High mobility group (HMG) proteins are intrinsically disordered nuclear non-histone chromosomal proteins that play an essential role in many biological processes by regulating the expression of numerous genes in eukaryote cells. HMGA proteins contain three DNA binding motifs, the “AT-hooks”, that bind preferentially to AT-rich sequences in the minor groove of B-form DNA. The AT-hook motif is formed by a short stretch of amino acids containing a conserved core sequence, Arg-Gly-Arg-Pro (R-G-R-P), flanked by other positively charged amino acids. HMGA are abundant nonhistone architectural nuclear factors that are involved in the modulation of chromatin structure and gene expression, thus influencing a vast array of biological processes including growth, proliferation, differentiation and death.

In the present study, we elucidate the crystal structure of the complex of AT-hook 1 (KRGRGRPRK) with the DNA oligonucleotide d(CGTTAATTAACG)2 at 1.40 Å resolution. Four Mg ions also contribute to stabilize the crystal structure. The terminal bases of the dodecamers do not form Watson-Crick base pairs; instead, the terminal guanines occupy an external position and form N2-N3 hydrogen bonds with the guanines from a neighbour stacked duplex. Peptide G is fully visible in the structure. It has the conformation expected for an AT-hook; its R3-G4 region enters into the minor groove of the AT region of the EF oligonucleotide duplex. Also, the neighbouring K2 and R5 residues interact with EF phosphates and increase the stability of this AT-hook 1. The rest of the peptide extends away and shows ionic interactions with the CD oligonucleotide duplex. In summary, two peptides and two oligonucleotide duplexes present clear AT hooks: peptide G with chains E-F and chains C-D, and peptide H with chains A-B. The other I peptide stabilizes A-B and E-F oligonucleotide duplexes by ionic interactions. In contrast to AT-hook 3 which bends DNA and shows a larger minor groove widening, AT-hook 1 binds neighbouring DNA molecules and displays moderate widening of DNA upon binding.

>[3x]XKRGRGRPRK> MAQMTMVQAITDALRIELKNDPNVLIFGEDVG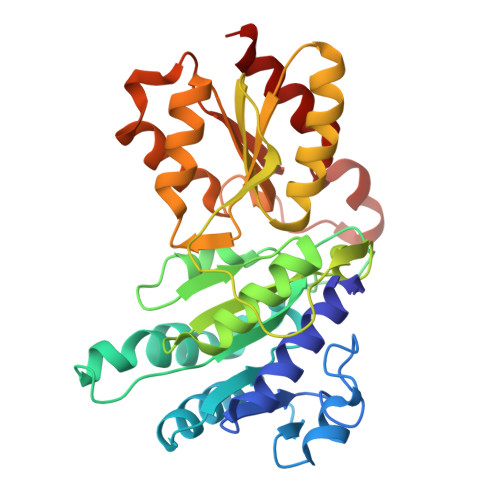VNGGVFRATEGLQAEFGEDRVFDTPLAESGIGGLAIGLALQGFRPVPEIQFFGFVYEVMDSICGQMARIRYRTGGRYHMPITIRSPFGGGVHTPELHSDSLEGLVAQQPGLKVVIPSTPYDAKGLLISAIRDNDPVIFLEHLKLYRSFRQEVPEGEYTIPIGKADIKREGKDITIIAYGAMVHESLKAAAELEKEGISAEVVDLRTVQPLDIETIIGSVEKTGRAIVVQEAQRQAGIAANVVAEINERAILSLEAPVLRVAAPDTVYPFAQAESVWLPNFKDVIETAKKVMNF> HHHHHHDLVE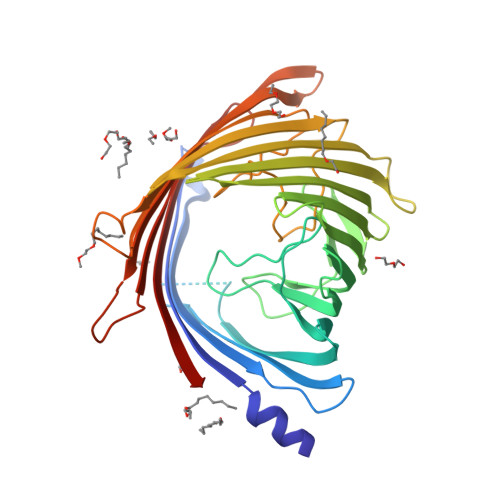DSHASLELRNFYFNRDFRQSGARDNADEWAQGFLLRLESGFSEGTVGFGVDAIGLLGFKLDSGSGSGGTGLLPADGSAGGSQDDYAKLGLTAKARVSNSLLKVGALHFKSPLVSANDTRLLPELFRGALLDVQEIDGLTLRGAHLDRNKLNSSSDYQVFSANRIGGRSDAFDFAGGDYRLTPALTASLHQGRLKDIYRQTFAGLVHTLDLGGQRSLKSDLRFARASEDGGFRELDNRAFGALFSLRLGAHAVAAGYQRISGDDPYPYIAGSDPYLVNFIQIGDFGNVDERSWQLRYDYDFGALGLPGLSFMSRYVSGDNVARGAANDGKEWERNTDLGYVVQSGPLKNLGVKWRNATVRSNFANDLDENRLILSYSLALW>MLTNSEKSRFFLADLTGEVQSIPNTYGYISGLGLFRSAPQTQTTFLMDLTDWDISLLDAVDRTSRKAETSAPERVRQISFPMMYFKEVESITPDEIQGVRQPGTANELTTEAVVRAKKLMKIRTKFDITREFLFMQALKGKVIDANGVLYADLYKQFDVTKKTIYFDLDNPNSDIDAHIEDLRMHMEDEAKTGTVINGEEIHIVVDRTFFSKLIKHPKIRDAYLAQQTPLAWQQITGSLRTGGTDGVQAHMNRFYYGGVVFVQYNGKFKDKRGKTHTLVSIDGVSDTNVGVGHAFPNVAMLGEANNIFEVAYAPCPKMGYANTLGQELYVFEYEKDRDEGIDFEAHSYMLPYCTRPQLLVDVRSDAE[9x];>[9x]MAYQGFTKLGEREPLNDIILWEEITPTGHSRKEYAPVASTEYRVGEVLKADGSKVAAGQEAQADSVCIVNFYADLQLSYHGQLKVVGIYRDAELKDLLKLESGVDAAAVKSALKAKGIDFVPTGL;> MIKAKTYPDFKEFVKDFVANVKAGKRYDFRKYQEAVLPLTYSSPWPESDIPEVTDFNYTPDYTVPFSEELLYSVGAQMRTADFFMDLQYAIINGKDVDTVYCEWLARVKPFSMLNAKLKDSAQPPVITTQPTGGAVNEGSAINLSIVATNATSYQWKKGSSDISGATSATYTKAGAVPADAGSYTCVVTNDVGSTTSDAAVITINPLPVITTQPTSKAVNESSTLTLSVVATGATSYQWKKNGTNISGATSATYSKANAKTTDAGSYTCVVTNAVGSVTSNAATVTINPLPVITVQPQDQDLTVGQTLTISITATGATGYQWRKGNSNISGATSATYTKASVTTADDGNYDCVVTNAVGSVTSHQAKVQVTA

Bacteriophage Sf14 infects the human pathogen Shigella flexneri. Here, we report multiple high-resolution structures of the full Sf14 particle, including symmetric and asymmetric reconstructions of the virion capsid, empty capsid, portal region, tail, and baseplate. Sf14 virions have a spherical icosahedral capsid of 820 Å in diameter, which is connected to a long, contractile tail that is approximately 1205 Å long and an average of 235 Å in diameter, expanding to 315 Å at the baseplate. Overall, phage Sf14 appears to share some similarities to other model phages, but in different combinations: both λ- and T4-like decoration proteins, HK97-like capsid and portal proteins, T4/Mu-like tail fibers, a Mu-like baseplate, and a P2-like tail needle.

In addition to the virion capsid, we determined the structure of spontaneous empty capsids, which have a mixture of non-attached or attached tails, the latter of which are contracted or non-contracted, but contain no genome. These particles are prevalent in typical Sf14 preparations and were hypothesized to be destabilized capsids lacking at least one decoration protein. However, these proteins are still present in the empty capsids and the etiology of these particles remains elusive. We hypothesized that the large proportion of empty capsids could be due to a loss of one or both decoration proteins. However, after resolving a separate structure based on empty particles alone, we did not see observable differences in the capsid composition or conformation. Results shown here are consistent with this hypothesis, as even degraded capsids without genome still contain both decoration proteins. The gp33 decoration proteins may be serving another function, such as host attachment or particle aggregation, or they may stabilize the capsid during DNA packaging but subsequently lose the genome through weakness elsewhere.> GSHMSQATSQPINFQVQADGSSEKSHMDDYMQHPGKVIKQNNKYYFQTVLNNASFWKEYKFYNANNQELATTVVNDNKKADTRTINVAVE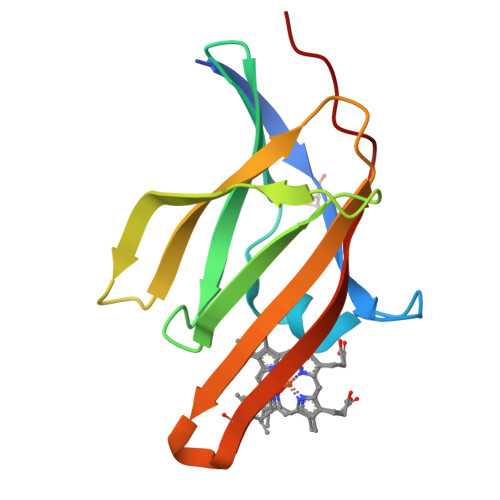PGYKSLTTKVHIVVPQINYNHRYTTHLEFEKAIPTLA> MPDPAAHLPFFYGSISRAEAEEHLKLAGMADGLFLLRQCLRSLGGYVLSLVHDVRFHHFPIERQLNGTYAIAGGKAHCGPAELCEFYSRDPDGLPCNLRKPCNRPSGLEPQPGVFDCLRDAMVRDYVRQTWKLEGEALEQAIISQAPQVEKLIATTAHERMPWYHSSLTREEAERKLYSGAQTDGKFLLRPRKEQGTYALSLIYGKTVYHYLISQDKAGKYCIPEGTKFDTLWQLVEYLKLKADGLIYCLKEACPNSSASNASGAAAPTLPAHPSTLTHPQRRIDTLNSDGYTPEPARITSPDKPRPMPMDTSVFESPFSDPEELKDKKLFLKRDNLLIADIELGCGNFGSVRQGVYRMRKKQIDVAIKVLKQGTEKADTEEMMREAQIMHQLDNPYIVRLIGVCQAEALMLVMEMAGGGPLHKFLVGKREEIPVSNVAELLHQVSMGMKYLEEKNFVHRNLAARNVLLVNRHYAKISDFGLSKALGADDSYYTARSAGKWPLKWYAPECINFRKFSSRSDVWSYGVTMWEALSYGQKPYKKMKGPEVMAFIEQGKRMECPPECPPELYALMSDCWIYKWEDRPDFLTVEQRMRACYYSLASKVEGGSA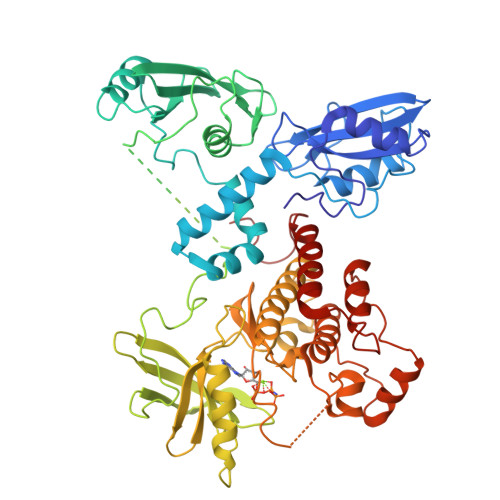LEVA>MSVLVPMVVEQTSRGERAYDIYSRLLKDRVIFLVGQVEDHMANLAIAQMLFLES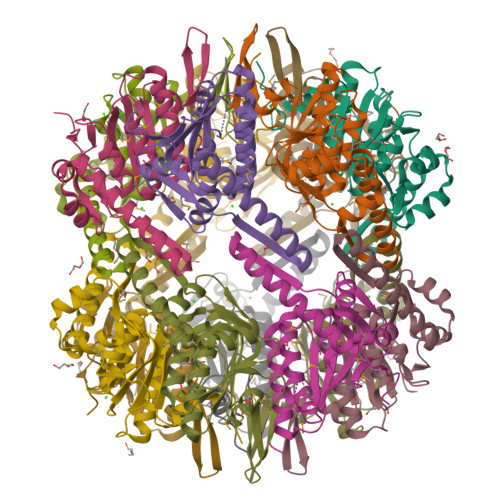ENPNKDINLYINSPGGAVTSAMAIYDTMQFVKPDVRTLCIGQAASAGALLLAGGAKGKRHCLPHSSVMIHQVLGGYQGQGTDIQIHAKQTQRVSDQLNQILAKHTGKDIERVEKDTNRDYFLTPEEAVEYGLIDSIFKERP[14x]> GSHMAARTDNSIVVNAPFELVWDVTNDIEAWPELFSEYAEAEILRQDGDGFDFRLKTRPDANGRVWEWVSHRVPDKGSRTVRAHRVETGPFAYMNLHWTYRAVAGGTEMRWVQEFD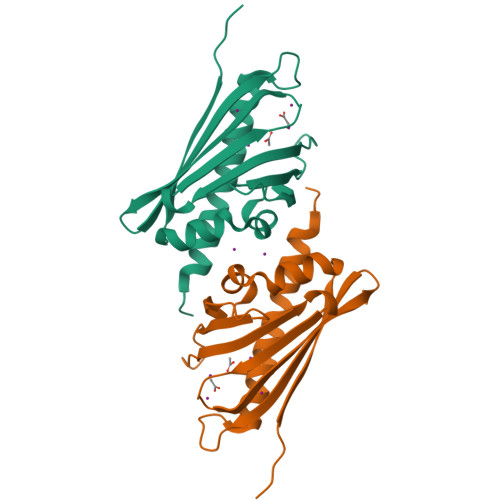MKPGAPFDNAHMTAHLNTTTRANMERIKKIIEDRHREGQRT> GSEDTMDRINKDHDHTTSVASRFILADVITSTAFSNASGDINTYASSYIEYEVGVDNQLYYAEVRENEPSSSSTFNNSWNGIYSSLKNARIIIDQCGEG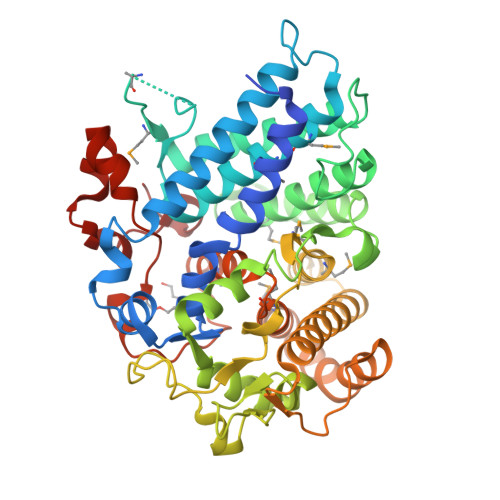GRDHGNDVTRGMAEVMAAYNCALIADFFGDAPCSQAALVDEKGSPVYMTPKMDTQQEIYTQIISYLDDAIANLQKEDLADVTEQDFLYAGDADKWLKFAYGLKARYTMRLINRSSNKSADYEKVLDYVSKSFTSADDQAAFDIYDSNNINPFYGFYNSRAGFGASTSLGTKLLAYNDPRANRAFFTPIVDKKRSQVAANDPSLVPAPNGSPDQSTSKYGISAFVYAKTAPTLLMSYHELMFLKAEALCRLNRDAEDALKEAVVAGLLNAENSISIAIKELGSGLNTNSSEVITETSAGKYFDDVVKAKYAANPLQETMIQKYLAMWGASGEATETYNDFRRMKGLNENFITLTNPNNSSKFPLRYPYGNSDTAANPEVKAAYGNGDYVYSEPVWWAGGSR Mofezolac | C19 H17 N 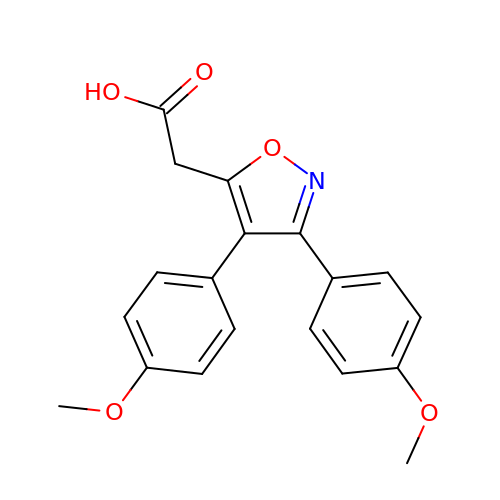O5 | DJEIHHYCDCTAAH-UHFFFAOYSA-N CIS-[4,5-BIS-(4-BROMOPHENYL)-2-(2-ETHOXY-4-METHOXYPHENYL)-4,5-DIHYDROIMIDAZOL-1-YL]-[4-(2-HYDROXYETHYL)PIPERAZIN-1-YL]METHANONE 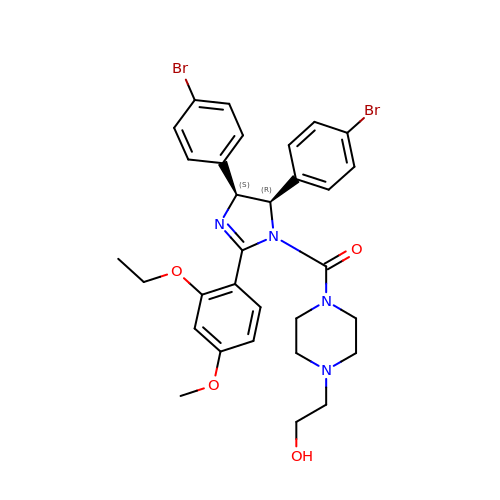| C31 H34 Br2 N4 O4 | PVRYEWOXWGDQHA-URLMMPGGSA-N>[2x]NARKVQMGAKDATPVPCGRWAKILEKDKRTQQMRMQRLKAKLQMPFQSGEFKALTRRLQVEPRLLSKQMAGCLEDCTRQAPESPWEEQLARLLQEAPGKLSLDVEQAPSGQHSQAQLSGQQQRLLAFFKCCLLTDQLPLAHHLLVVHHGQRQKRKLLTLDMYNAVMLGWARQGAFKELVYVLFMVKDAGLTPDLLSYAAALQCMGRQDQDAGTIERCLEQMSQEGLKLQALFTAVLLSEEDRATVLKAVHKVKPTFSLPPQLPPPVNTSKLLRDVYAKDGRVSYPKLHLPLKTLQCLFEKQLHMELASRVCVVSVEKPTLPSKEVKHARKTLKTLRDQWEKALCRALRETKNRLEREVYEGRFSLYPFLCLLDEREVVRMLLQVLQALPAQGESFTTLARELSARTFSRHVVQRQRVSGQVQALQNHYRKYLCLLASDAEVPEPCLPRQYWEALGAPEALREQPWPLPVQMELGKLLAEMLVQATQMPCSLDKPHRSSRLVPVLYHVYSFRNVQQIGILKPHPAYVQLLEKAAEPTLTFEAVDVPMLCPPLPWTSPHSGAFLLSPTKLMRTVEGATQHQELLETCPPTALHGALDALTQLGNCAWRVNGRVLDLVLQLFQAKGCPQLGVPAPPSEAPQPPEAHLPHSAAPARKAELRRELAHCQKVAREMHSLRAEALYRLSLAQHLRDRVFWLPHNMDFRGRTYPCPPHFNHLGSDVARALLEFAQGRPLGPHGLDWLKIHLVNLTGLKKREPLRKRLAFAEEVMDDILDSADQPLTGRKWWMGAEEPWQTLACCMEVANAVRASDPAAYVSHLPVHQDGSCNGLQHYAALGRDSVGAASVNLEPSDVPQDVYSGVAAQVEVFRRQDAQRGMRVAQVLEGFITRKVVKQTVMTVVYGVTRYGGRLQIEKRLRELSDF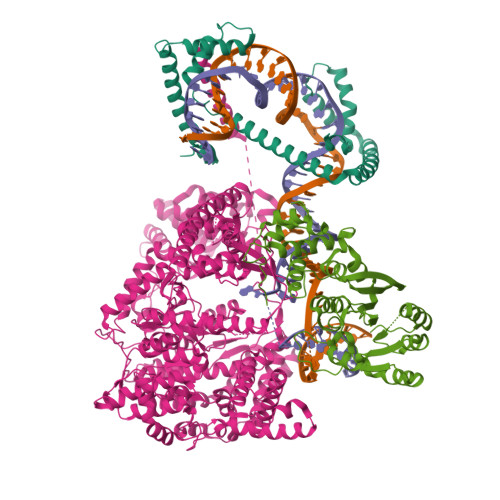PQEFVWEASHYLVRQVFKSLQEMFSGTRAIQHWLTESARLISHMGSVVEWVTPLGVPVIQPYRLDSKVKQIGGGIQSITYTHNGDISRKPNTRKQKNGFPPNFIHSLDSSHMMLTALHCYRKGLTFVSVHDCYWTHAADVSVMNQVCREQFVRLHSEPILQDLSRFLVKRFCSEPQKILEASQLKETLQAVPKPGAFDLEQVKRSTYFFS;>NASSVLASSPKKPVSSYLRFSKEQLPIFKAQNPDAKTTELIRRIAQRWRELPDSKKKIYQDAYRAEWQVYKEEISRFKEQLTPSQIMSLEKEIMDKHLKRKAMTKKKELTLLGKPKRPRSAYNVYVAERFQEAKGDSPQEKLKTVKENWKNLSDSEKELYIQHAKEDETRYHNEMKSWEEQMIEVGRKDLLRRTIKKQRKYGAEE[2x];>NARFCILGSEAATRKHLPARNHCGLSDSSPQLWPEPDFRNPPRKASKASLDFKRYVTDRRLAETLAQIYLGKPSRPPHLLLECNPGPGILTQALLEAGAKVVALESDKTFIPHLESLGKNLDGKLRVIHCDFFKLDPRSGGVIKPPAMSSRGLFKNLGIEAVPWTADIPLKVVGMFPSRGEKRALWKLAYDLYSCTSIYKFGRIEVNMFIGEKEFQKLMADPGNPDLYHVLSVIWQLACEIKVLHMEPWSSFDIYTRKGPLENPKRRELLDQLQQKLYLIQMIPRQNLFTKNLTPMNYNIFFHLLKHCFGRRSATVIDHLRSLTPLDARDILMQIGKQEDEKVVNMHPQDFKTLFETIERSKDCAYKWLYDETLEDR[2x]> SSKNEWRKSAIANTLLYLRLKNIYVSADDFVEEQNVYVLPKNLLKKFIEISDVKIQVAAFIYGM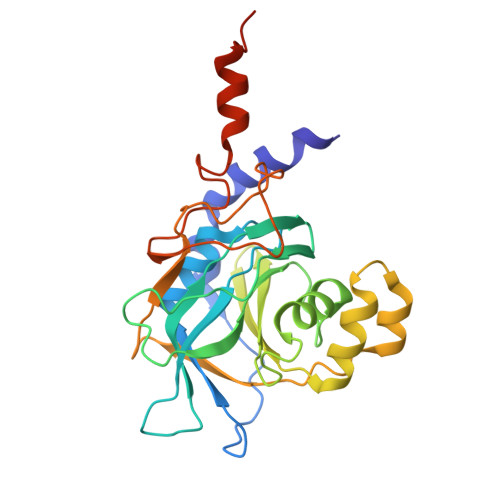SAKDHPKVKEIKTVVLVPQLGHVGSVQISNIPDIGDLPDTEGLELLGWIHTQTEELKFMAASEVATHSKLFADKKRDCIDISIFSTPGSVSLSAYNLTDEGYQWGEENKDIMNVLSEGFEPTFSTHAQLLLSDRITGNFIIPSGNVWNYTFMGTAFNQEGDYNFKYGIPLEFYNEMHRPVHFLQFSELAGDEELEAEQIDVFS γ-Glutamyltranspeptidase (GGT) is an enzyme that plays a central role in glutathione metabolism, and acivicin is a classical inhibitor of GGT. GGT is a heterodimeric enzyme consisting of large (L; ∼40 kDa) and small (S; ∼20 kDa) subunits that are formed from an inactive precursor protein (∼60 kDa) by post-translational and autocatalytic cleavage. The autocatalytic processing requires a specific nucleophilic residue (Thr) that catalyzes the cleavage of the peptide bond just preceding this residue to liberate the catalytic S subunit with this residue at its N-­terminus. Bacterial GGTs share the same overall fold, but B. subtilis GGT is unique in that it lacks a lid-loop that covers the bound substrate and has a tail at the C-terminal end of the L subunit.

To gain insights into the binding affinity of the acivicin moiety, we assessed the electron-density maps after soaking the GGT crystals in acivicin solution for various soaking times and trapping its binding processes by flash-cooling. A similar vague electron density was also observed in the substrate-free E. coli GGT structure. The differences are discussed in terms of the recognition of the α-­amino and α-carboxy groups in preference to the dihydro­isoxazole ring, as observed in time-lapse soaking crystal structures of B. subtilis GGT with acivicin.

> MNHKVHHHHHHIEGRHMKRTWNVCLTALLSVLLVAGSVPFHAEAKKPPKSYDEYKQVDVGKDGMVATAHPLASEIGADVLKKGGNAIDAAVAIQFALNVTEPMMSGIGGGGFMMVYDGKTKDTTIIDSRERAPAGATPDMFLDENGKAIPFSERVTKGTAVGVPGTLKGLEEALDKWGTRSMKQLITPSIKLAEKGFPIDSVLAEAISDYQEKLSRTAAKDVFLPNGEPLKEGDTLIQKDLAKTFKLIRSKGTDAFYKGKFAKTLSDTVQDFGGSMTEKDLENYDITIDEPIWGDYQGYQIATTPPPSSGGIFLLQMLKILDHFNLSQYDVRSWEKYQLLAETMHLSYADRASYAGDPEFVNVPLKGLLHPDYIKERQQLINLDQVNKKPKAGDPWKYQEGSANYKQVEQPKDKVEGQ;> TTHFTVADRWGNVVSYTTTIEQLFGTGIMVPDYGVILNNELTDFDAIPGGANEVQPNKRPLSSMTPTILFKDDKPVLTVGSPGGATIISSVLQTILYHIEYGMELKAAVEEPRIYTNSMSSYRYEDGVPKDVLSKLNGMGHKFGTSPVDIGNVQSISIDHENGTFKGVADSSRNGAAIGINLKRK> AEGQTNADDTLVVEASTPSLYAPQQSADPKFSRPVADTTRTMTVISEQVIKDQGATNLTDALKNVPGVGAFFAGENGNSTTGDAIYMRGADTSNSIYIDGIRDIGSVSRDTFNTEQVEVIKGPSGTDYGRSAPTGSINMISKQPRNDSGIDASASIGSAWFRRGTLDVNQVIGDTTAVRLNVMGEKTHDAGRDKVKNERYGVAPSVAFGLGTANRLYLNYLHVTQHNTPDGGIPTIGLPGYSAPSAGTAALNHSGKVDTHNFYGTDSDYDDSTTDTATMRFEHDINDNTTIRNTTRWSRVKQDYLMTAIMGGASNITQPTSDVNSWTWSRTANTKDVSNKILTN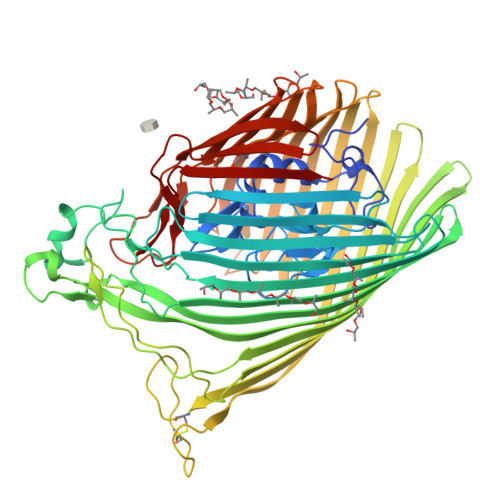QTNLTSTFYTGSIGHDVSTGVEFTRETQTNYGVNPVTLPAVNIYHPDSSIHPGGLTRNGANANGQTDTFAIYAFDTLQITRDFELNGGIRLDNYHTEYDSATACGGSGRGAITCPTGVAKGSPVTTVDTAKSGNLMNWKAGALYHLTENGNVYINYAVSQQPPGGNNFALAQSGSGNSANRTDFKPQKANTSEIGTKWQVLDKRLLLTAALFRTDIENEVEQNDDGTYSQYGKKRVEGYEISVAGNITPAWQVIGGYTQQKATIKNGKDVAQDGSSSLPYTPEHAFTLWSQYQATDDISVGAGARYIGSMHKGSDGAVGTPAFTEGYWVADAKLGYRVNRNLDFQLNVYNLFDTDYVASINKSGYRYHPGEPRTFLLTANMHF>[12x]SRVPSPPPPAEMSSGPV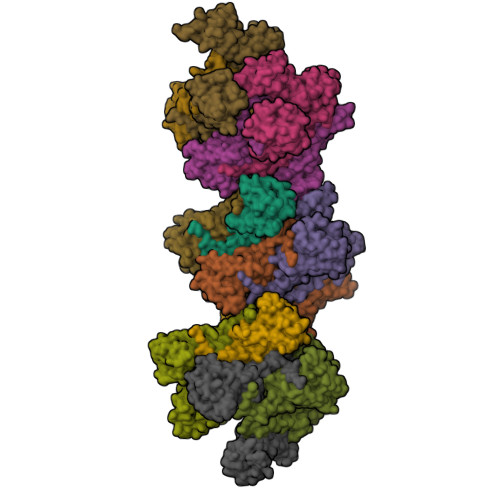AESRCYTQIKVVKFSYMWTINNFSFCREEMGEVIKSSTFSSGANDKLKWCLRVNPKGLDEESKDYLSLYLLLVSCPKSEVRAKFKFSILNAKGEETKAMESQRAYRFVQGKDWGFKKFIRRDFLLDEANGLLPDDKLTLFCEVSVVQDSVNISGQNTMNMVKVPECRLADELGGLWENSRFTDCCLCVAGQEFQAHKAILAARSPVFSAMFEHEMEESKKNRVEINDVEPEVFKEMMCFIYTGKAPNLDKMADDLLAAADKYALERLKVMCEDALCSNLSVENAAEILILADLHSADQLKTQAVDFINYHASDVLETSGWKSMVVSHPHLVAEAYRSLASAQCPFLGPPRKRLKQS>[4x]MLQDPIPAKIYDKNGELVKTLDNGQRHEHVNLKDVPKSMKDAVLATEDNRFYEHGALDYKRLFGAIGKNLTGGFGSEGASTLTQQVVKDAFLSQHKSIGRKAQEAYLSYRLEQEYSKDDIFQVYLNKIYYSDGVTGIKAAAKYYFNKDLKDLNLAEEAYLAGLPQVPNNYNIYDHPKAAEDRKNTVLYLMHYHKRITDKQWEDAKKIDLKANLVNRTPEERQNIDTNQDSEYNSYVNFVKSELMNNKAFKDENLGNVLQSGIKIYTNMDKDVQKTLQNDVDNGSFYKNKDQQVGATILDSKTGGLVAISGGRDFKDVVNRNQATDPHPTGSSLKPFLAYGPAIENMKWATNHAIQDESSYQVDGSTFRNYDTKSHGTVSIYDALRQSFNIPALKAWQSVKQNAGNDAPKKFAAKLGLNYEGDIGPSEVLGGS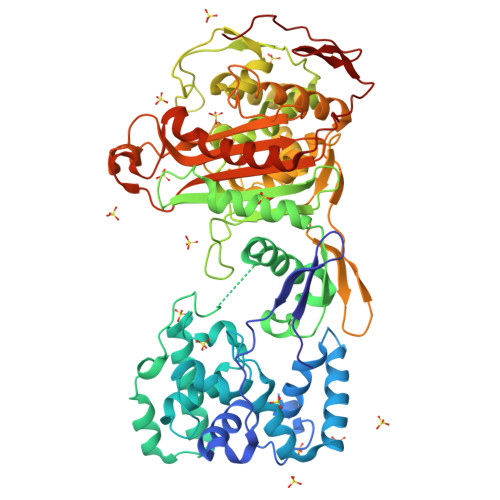ASEFSPTQLASAFAAIANGGTYNNAHSIQKVVTRDGETIEYDHTSHKAMSDYTAYMLAEMLKGTFKPYGSAYGHGVSGVNMGAKTGTGTYGAETYSQYNLPDNAAKDVWINGFTPQYTMSVWMGFSKVKQYGENSFVGHSQQEYPQFLYENVMSKISSRDGEDFKRPSSVSGSIPSINVSGSQDNNTTNRSTH> MNITVELTFFEPYRLVEWFDWDARKKSHSAMRGQAFAQWTWKGKGRTAGKSFITGTLVRSAVIKAVEELLSLNNGKWEGVPCCNGSFQTDESKGKKPSFLRKRHTLQWQANNKNICDKEEACPFCILLGRFDNAGKVHERNKDYDIHFSNFDLDHKQEKNDLRLVDIASGRILNRVDFDTGKAKDYFRTWEADYETYGTYTGRITLRNEHAKKLLLASLGFVDKLCGALCRIEVIKKSESPLPSDTKEQSYTKDDTVEVLSEDHNDELRKQAEVIVEAFKQNDKLEKIRILADAIRTLRLHGEGVIEKDELPDGKEERDKGHHLWDIKVQGTALRTKLKELWQSNKDIGWRKFTEMLGSNLYLIYKKETGGVSTRFRILGDTEYYSKAHDSEGSDLFIPVTPPEGIETKEWIIVGRLKAATPFYFGVQQPSDSIPGKEKKSEDSLVINEHTSFNILLDKENRYRIPRSALRGALRRDLRTAFGSGCNVSLGGQILCNCKVCIEMRRITLKDSVSDFSEPPEIRYRIAKNPGTATVEDGSLFDIEVGPEGLTFPFVLRYRGHKFPEQLSSVIRYWEENDGKNGMAWLGGLDSTGKGRFALKDIKIFEWDLNQKINEYIKERGMRGKEKELLEMGESSLPDGLIPYKFFEERECLFPYKENLKP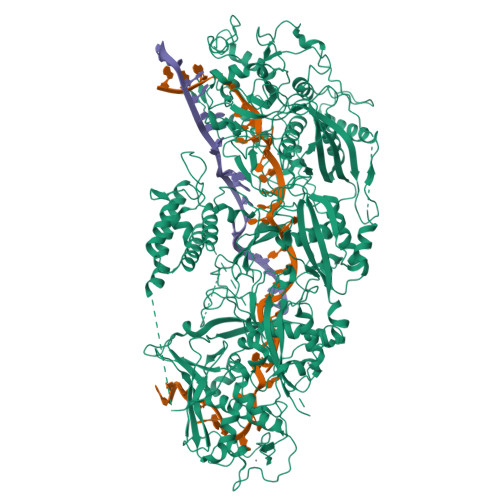QWSEVQYTIEVGSPLLTADTISALTEPGNRDAIAYKKRVYNDGNNAIEPEPRFAVKSETHRGIFRTAVGRRTGDLGKEDHEDCTCDMCIIFGNEHESSKIRFEDLELINGNEFEKLEKHIDHVAIDRFTGGALDKAKFDTYPLAGSPKKPLKLKGRFWIKKGFSGDHKLLITTALSDIRDGLYPLGSKGGVGYGWVAGISIDDNVPDDFKEMINKTEMPLPEEVEESNNGPINNDYVHPGHQSPKQDHKNKNIYYPHYFLDSGSKVYREKDIITHEEFTEELLSGKINCKLETLTPLIIPDTSDENGLKLQGNKPGHKNYKFFNINGELMIPGSELRGMLRTHFEALTKSCFAIFGEDSTLSWRMNADEKDYKIDSNSIRKMESQRNPKYRIPDELQKELRNSGNGLFNRLYTSERRFWSDVSNKFENSIDYKREILRCAGRPKNYKGGIIRQRKDSLMAEELKVHRLPLYDNFDIPDSAYKANDHCRKSATCSTSRGCRERFTCGIKVRDKNRVFLNAANNNRQYLNNIKKSNHDLYLQYLKGEKKIRFNSKVITGSERSPIDVIAELNERGRQTGFIKLSGLNNSNKSQGNTGTTFNSGWDRFELNILLDDLETRPSKSDYPRPRLLFTKDQYEYNITKRCERVFEIDKGNKTGYPVDDQIKKNYEDILDSYDGIKDQEVAERFDTFTRGSKLKVGDLVYFHIDGDNKIDSLIPVRISRKCASKTLGGKLDKALHPCTGLSDGLCPGCHLFGTTDYKGRVKFGFAKYENGPEWLITRGNNPERSLTLGVLESPRPAFSIPDDESEIPGRKFYLHHNGWRIIRQKQLEIRETVQPERNVTTEVMDKGNVFSFDVKFENLREWELGLLLQSLDPGKNIAHKLGKGKPYGFGSVKIKIDSLHTFKINSNNDKIKRVPQSDIREYINKGYQKLIEWSGNNSIQKGNVLPQWHVIPHIDKLYKLLWVPFLNDSKLEPDVRYPVLNEESKGYIEGSDYTYKKLGDKDNLPYKTRVKGLTTPWSPWNPFQVIAEHEEQEVNVTGSRPSVTDKIERDGKMV>[2x]MPNHLTLEQISLFKQLPGYWGCKDLNSVF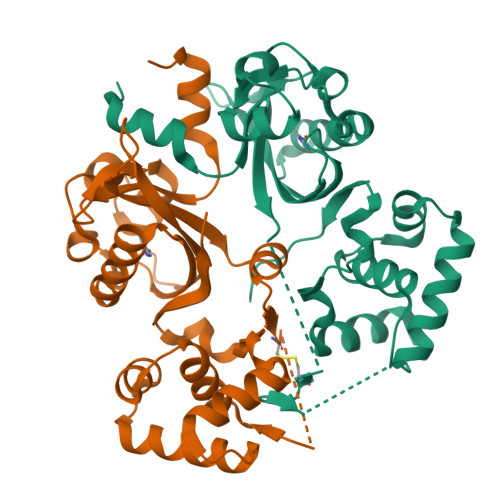VYANQAYGELIGLKRAEDCIGRTDFEMPSPTAACAAEFQQQDRYVIETGHSVKVLDIHPYPDGHWHAHIFTKTPWRDSQGKIQGTIFFGQDLTDTAILEVGHWVCRATGLSTSTTFKSVADRDTLKLTARESEVLFLLLYGKKPQHIARVMGISIKTVEGYEAKLRSKFGALSKDQLIDLALDRGFGSVIPKTLLRKQLSVVLSDHTIPKKVDVVAQ Proteins containing a FIC domain catalyze AMPylation and other post-translational modifications (PTMs). Among these, Bartonella effector proteins (Beps) comprise a particularly diverse ensemble of FIC domains that subvert various host cellular functions. The FIC fold comprises eight conserved α-helices and encompasses a characteristic active site loop between helices α4 and α5 that forms most of the catalytic center and the substrate binding pocket. Additionally, FIC domains generally contain a β-hairpin between helix α2 and helix α3 that is referred to as the “flap” and mediates docking of a target segment in extended conformation via β-strand augmentation.

The structures of Bhe_BepA, Bcl_Bep1, Bqu_BepC, and Btr_BepC exhibit all features defining a FIC AMP transferase as described in the first chapter and elsewhere. However, BepC proteins are special in that they have a lysine instead of a Mg2+-coordinating aspartate/glutamate in the FIC motif. Thus, BepC proteins appear to require no divalent cation for substrate binding, in contrast to all FIC AMP transferases characterized so far. For the FIC domain of BepC with its non-canonical FIC signature motif, no enzymatic activity has been found although it binds to the RhoGEF GEF-H1 and activates this signaling protein by relocalization to the plasma membrane. For BepC, despite its canonical signature motif, no catalytic activity has yet been found, but its BepFIC domain mediates protein–protein interaction with the RhoGEF GEF-H1, thereby activating RhoA signaling. Bqu_BepC FIC crystals were grown from a solution of 10% w/v PEG 4000, 20% v/v glycerol, 0.1 M bicine/Trizma base, pH 8.5, and 0.03 M each of NaF, NaBr, and NaI. Data for Bqu_BepC FIC, B15_Bep8 FIC, and Bcl_Bep5 FIC were collected at 100 K on a Rayonix MX-300 detector at a wavelength of 0.9786 Å on beamline 21-ID-G at the Advanced Photon Source (APS, Argonne, IL, USA).

>[2x]MAHHHHHHMEHNYFYKNSATLKNKHGIKNPRKLYERCAHETAREAVNFRLEPPPGKFDAAYLRTIHWCLFHNTFEWAGVTRDQPFTFEDGSTACMPAMRPKGYKVPFAVGSQIQRELKKLEQRLTAKNNLQGLSRQEFAANAAEVFTALDHAHPFRKGNGRTQRMFMEKLGQAAGYKIDFSLITKERMTYASIEAMQHNNPEPMKDLFEDITHPQKSLLLKEFISQM>MVEHDKSGSKRQELRSNMRNLITLNKGKFKPTASTAEGDEDDLSFTLLDSVFDTLSDSITCVLGSTDIGAIEVQQFMKDGSRNVLASFNIQTFDDKLLSFVHFADINQLVFVFEQGDIITATYDPVSLDPAETLIEIMGTIDNGIAAAQWSYDEETLAMVTKDRNVVVLSKLFEPISEYHLEVDDLKISKHVTVGWGKKETQFRGKGARAMEREALASLKASGLVGNQLRDPTMPYMVDTGDVTALDSHEITISWRGDCDYFAVSSVEEVPDEDDETKSIKRRAFRVFSREGQLDSASEPVTGMEHQLSWKPQGSLIASIQRKTDLGEEDSVDVIFFERNGLRHGEFDTRLPLDEKVESVCWNSNSEALAVVLANRIQLWTSKNYHWYLKQELYASDISYVKWHPEKDFTLMFSDAGFINIVDFAYKMAQGPTLEPFDNGTSLVVDGRTVNITPLALANVPPPMYYRDFETPGNVLDVACSFSNEIYAAINKDVLIFAAVPSIEEMKKGKHPSIVCEFPKSEFTSEVDSLRQVAFINDSIVGVLLDTDNLSRIALLDIQDITQPTLITIVEVYDKIVLLRSDFDYNHLVYETRDGTVCQLDAEGQLMEITKFPQLVRDFRVKRVHNTSAEDDDNWSAESSELVAFGITNNGKLFANQVLLASAVTSLEITDSFLLFTTAQHNLQFVHLNSTDFKPLPLVEEGVEDERVRAIERGSILVSVIPSKSSVVLQATRGNLETIYPRIMVLAEVRKNIMAKRYKEAFIVCRTHRINLDILHDYAPELFIENLEVFINQIGRVDYLNLFISCLSEDDVTKTKYKETLYSGISKSFGMEPAPLTEMQIYMKKKMFDPKTSKVNKICDAVLNVLLSNPEYKKKYLQTIITAYASQNPQNLSAALKLISELENSEEKDSCVTYLCFLQDVNVVYKSALSLYDVSLALLVAQKSQMDPREYLPFLQELQDNEPLRRKFLIDDYLGNYEKALEHLSEIDKDGNVSEEVIDYVESHDLYKHGLALYRYDSEKQNVIYNIYAKHLSSNQMYTDAAVAYEMLGKLKEAMGAYQSAKRWREAMSIAVQKFPEEVESVAEELISSLTFEHRYVDAADIQLEYLDNVKEAVALYCKAYRYDIASLVAIKAKKDELLEEVVDPGLGEGFGIIAELLADCKGQINSQLRRLRELRAKKEENPYAFYGQETEQADDVSVAPSETSTQESFFTRYTGKTGGTAKTGASRRTAKNKRREERKRARGKKGTIYEEEYLVQSVGRLIERLNQTKPDAVRVVEGLCRRNMREQAHQIQKNFVEVLDLLKANVKEIYSISEKDRERVNENGEVYYIPEIPVPEIHDFPKSHIVDF[2x];> MVECITPEAIFIGANKQTQVSDIHKVKKIVAFGAGKTIALWDPIEPNNKGVYATLKGHEAEVTCVRFVPDSDFMVSASEDHHVKIWKFTDYSHLQCIQTIQHYSKTIVALSALPSLISVGCADGTISIWRQNIQNDEFGLAHEFTIKKGFFYPLCLSLSKVEEKKYLLAIGGTNVNVFIASFILSDSGIEKCRVVAELEGHEDWVKSLAFRHQETPGDYLLCSGSQDRYIRLWRIRINDLIDDSEEDSKKLTLLSNKQYKFQIDDELRVGINFEALIMGHDDWISSLQWHESRLQLLAATADTSLMVWEPDETSGIWVCSLRLGEMSSKGASTATGSSGGFWSCLWFTHERMDFFLTNGKTGSWRMWATKDNIICDQRLGISGATKDVTDIAWSPSGEYLLATSLDQTTRLFAPWIYDASGRKREIATWHEFSRPQIHGYDMICVETVTDTRFVSGGDEKILRSFDLPKGVAGMLQKFVGIQFEEKSEMPDSATVPVLGLSNKAGEDDANEDDEEEEGGNKETPDITDPLSLLECPPMEDQLQRHLLWPEVEKLYGHGFEITCLDISPDQKLIASACRSNNVQNAVIRIFSTENWLEIKPALPFHSLTITRLKFSKDGKFLLSVCRDRKWALWERNMEDNTFELRFKNEKPHTRIIWDADWAPLEFGNVFVTASRDKTVKVWRHQKEPADDYVLEASIKHTKAVTAISIHDSMIREKILISVGLENGEIYLYSYTLGKFELITQLNEDITPADKITRLRWSHLKRNGKLFLGVGSSDLSTRIYSLAYE;> MARHGKGPKTNKKKLAPEKERFIQCCADITLELTDSLTSGTTREINLNGLITKYSKKYKLKQQPRLTDIINSIPDQYKKYLLPKLKAKPVRTASGIAVVAVMCKPHRCPHIAYTGNICVYCPGGPDSDFEYSTQSYTGYEPTSMRAIRARYDPYEQARGRVEQLKQLGHSIDKVEYVLMGGTFMSLPKEYREDFIVKLHNALSGFNGNDIDEAILYSQQSLTKCVGITIETRPDYCTQTHLDDMLKYGCTRLEIGVQSLYEDVARDTNRGHTVRSVCETFAVSKDAGYKVVSHMMPDLPNVGMERDIEQFKEYFENPDFRTDGLKIYPTLVIRGTGLYELWKTGRYKSYSANALVDLVARILALVPPWTRIYRVQRDIPMPLVTSGVDNGNLRELALARMKDLGTTCRDVRTREVGIQEVHHKVQPDQVELIRRDYYANGGWETFLSYEDPKKDILIGLLRLRKASKKYTYRKEFTSQRTSIVRELHVYGSVVPLHSRDPRKFQHQGFGTLLMEEAERIAKEEHGSEKISVISGVGVRNYYGKLGYELDGPYMSKRI;>[2x]MASSSHNPVILLKRILSLTESSPFILCLDSIAQTSYKLIQEFVHQSKSKGNEYPIVYISFETVNKPSYCTQFIDATQMDFVHLVKQIISYLPAATATQAKKHMVIIDSLNYISTEYITRFLSEIASPHCTMVATYHKDIKDENRTVIPDWNNNYPDKLTLLQFMATTIVDIDVVLTGTLDTEEVSELLNEFRIPRGLNNDIFQLRLVNKRKSGRSLEYDFIVNSNTHEYELLSTTKQEEESSSNGLETPEMLQGLTTFNLGTSNKQKLAKDQVALPFLEAQSFGQGGAIVYEYEKDDDYDEEDPYEDPF;>[2x]MGSVQRQDLVLFSDQSVLPAHFFQDSNSHNLFFITHQSCTQPLWMINALVETHVLGSPSSLNESSSSMLPSSTRSHAVLASFIHEQNYFTNSLNKLKIPSNNYNVLDFLSDFIVNNIHNKPRDKILSDVLAKFSAAIQNNPTDTIVIIEQPELLLSLVSGLTCSELNNKFITPLLRQCKVLIIVSNSDIFNIDEYDASVHSSNLQNFYKSSFIKSMINLNLNPLKTGFAKDVTGSLHVCRGGAPIATSNTSLHVVENEYLYLNEKESTKLFYR;>MSFRKRGEILNDRGSGLRGPLLRGPPRTSSTPLRTGNRRAPGNVPLSDTTARLKKLNIADESKTKMGLDSSHVGVRPSPATSQPTTSTGSADLDSILGHMGLPLGNSVLVEEQSTTEFHSILGKLFAAQGIVHNRISDSSADKTRNGDTHVIVLSLNQMFAKELPGIYKGSRKQMKKNLISEEESKVTVQNLNETQRSTPSRYKDLKIAWKYKLADEKRLGSPDRDDIQQNSEYKDYNHQFDITTRLMPAPIASELTFIAPTQPVSTILSQIEQTIKRNDKKLIRIVIPSLLHPAMYPPKMFESSEIIGLMHGVRSLVKKYYERVVLFASISIDIITPPLLVLLRNMFDSVINLEPFNQEMTEFLERVYKSQPGKIQHGLVHILKLPVFTDRGEMRVLKSEWAFKNGRKKFEIEQWGIPVDDAEGSAASEQSHSHSHSDEISHNIPAKKTKISLDY[2x]

In eukaryotes, wobble uridines are modified by Elongator, a large and highly conserved macromolecular complex. Elongator consists of two subcomplexes, namely Elp123 containing the enzymatically active Elp3 subunit and the associated Elp456 hetero-hexamer. The Elongator complex harbors two copies of each of its six subunits, namely Elongator proteins 1–6 (Elp1–Elp6). Decreased levels of wobble uridine modifications lead to ribosome pausing, incorrect protein folding and consequently trigger intracellular protein aggregation and proteotoxic stress.

Thereby, we determined the structure of ScElongator at an overall resolution of 4.35 Å. The reconstruction shows an additional, unambiguous density for the ScElp456 ring next to one of the two Elp123 lobes. Our Elongator cryo-EM structure reveals that the hetero-hexameric Elp456 occupies a position that faces the active site of Elp3 and bridges between the enzymatic subunit and the C-terminal region of Elp1. In detail, Elp123 and Elp456 subcomplexes interact with each other at three individual contact points involving Elp1, Elp3, Elp4, Elp5, and Elp6. The first contact point (CP1) is formed between less conserved residues of the Elp3 rSAM domain (Trp341 and Lys342) and a loop region in Elp4 (Tyr369, Ser371, Gln372, Lys375 and Glu401). The second contact point (CP2) is formed between a loop region of Elp4 (aa172-195) and helices α27 and α28 of the dimerization domain of Elp1 (Asp1160, Gln1164, Arg1171, Tyr1254, Arg1261 and Arg1265). The third contact point (CP3) is an interface that is created at the three-way junction between the KAT domain of Elp3 and the C-terminal residues of Elp6. Characteristic densities for the iron-sulfur cluster are clearly recognizable in both native and crosslinked structures of ScElongator. However, we were not able to identify densities for bound SAM or 5′-dA molecules, which were present in proximity to the cluster in the previous cryo-EM structure of the Elp123 subcomplex. In addition, our ScElongator model also clearly shows that the tRNA binding loop (aa1176–1251) of Elp1 is displaced by Elp456 and would not be able to interact with the T-arm of tRNAs.>TPRGFVVHTAPVGLADDGRDDFTVLASTAPATVSAVFTRSRFAGPSVVLCREAVADGQARGVVVLARNANVATGLEGEENAREVREAVARALGLPEGEMLIASTGVIGRQYPMESIREHLKTLEWPAGEGGFDRAARAIMTTDTRPKEVRVSVGGATLVGIAKGVGMLEPDMA[4x];>[4x]TLLTFFATDARLDPAEQDRLFRRVMDRTFNAVSIDTDTSTSDTAVLFANGLAGEVDAGEFEEALHTAALALVKDIASDGEGAAKLIEVQVTGARDDAQAKRVGKTVVNSPLVKTAVHGCDPNWGRVAMAIGKCSDDTD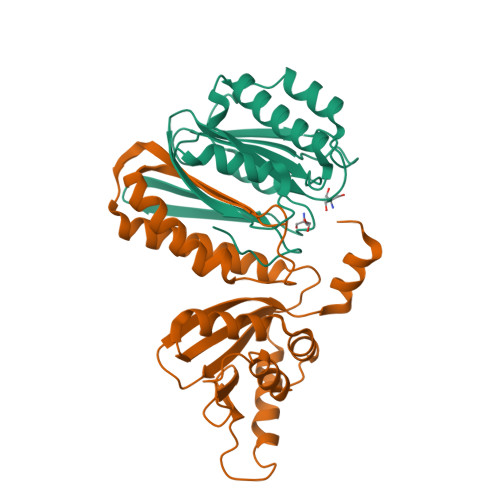IDQERVTIRFGEVEVYPPKARGDQADDALRAAVAEHLRGDEVVIGIDLAIADGAFTVYGCDLTEGYVRLNSEYTT1-(2-methyl-4-phenyl-pyrimidin-5-yl)-3-pyridin-2-yl-urea 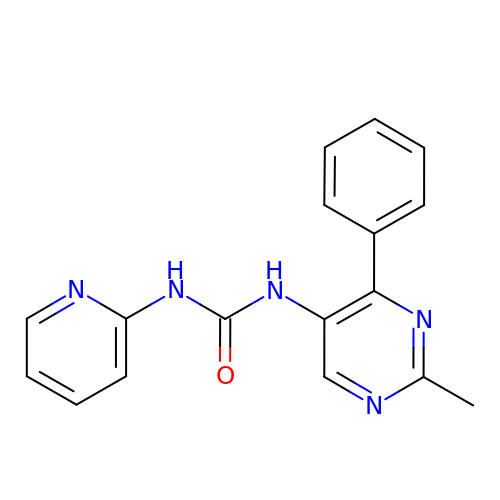| C17 H15 N5 O | NWPAIRZLGKDVNX-UHFFFAOYSA-N> ALVPMVIEQTSRGERSFDI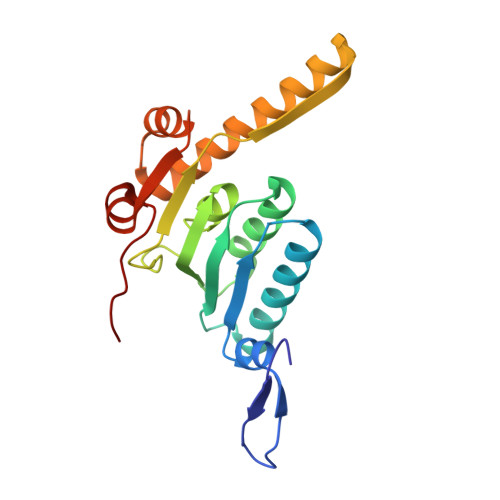YSRLLKERVIFLTGQVEDHMANLIVAQMLFLEAENPEKDIYLYINSPGGVITAGMSIYDTMQFIKPDVSTICMGQAASMGAFLLTAGAKGKRFCLPNSRVMIHQPLGGYQGQATDIEIHAREILKVKGRMNELMALHTGQSLEQIERDTERDRFLSAPEAVEYGLVDSILTHR>EMNSNVENLPPHIIRLVYKEVTTLTADPPDGIKVFPNEEDLTDLQVTIEGPEGTPYAGGLFRMKLLLGKDFPASPPKGYFLTKIFHPNVGANGEICVNVLKRDWTAELGIRHVLLTIKALLIHPNPESALNEEAGRL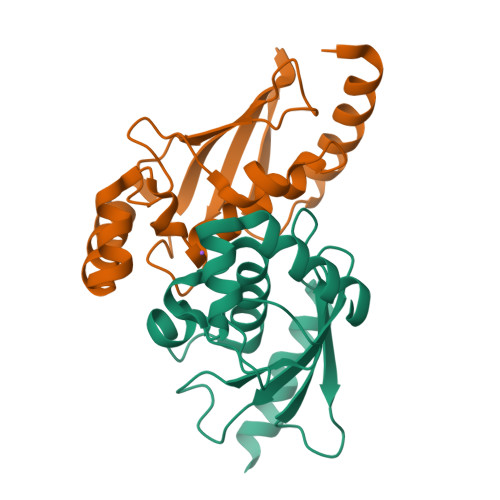LLENYEEYAARARLLTEIHG[2x]> HHHHHHSSGLVPRGSH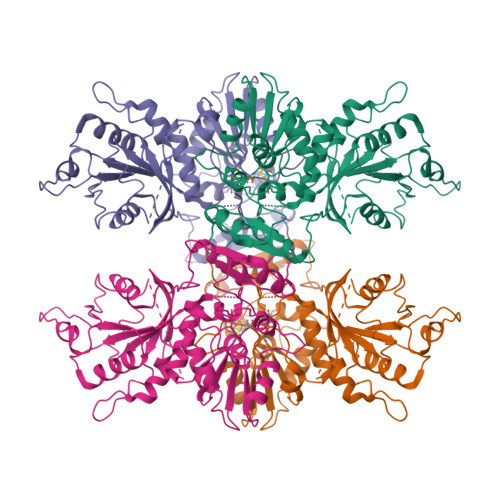MLEDPRRYTMRLPDAGFRRYIVVAGRRNVGKSSFMNALVGQNVSIVSDYAGTTTDPVYKSMELHPIGPVTLVDTPGLDDVGELGRLRVEKARRVFYRADCGILVTDSAPTPYEDDVVNLFKEMEIPFVVVVNKIDVLGEKAEELKGLYESRYEAKVLLVSALQKKGFDDIGKTISEILPGDEEIPYLGDLIDGGDLVILVVPIDLGAPKGRLIMPQVHAIREALDREAIALVVKERELRYVMENIGMKPKLVITDSQVAMKVASDVPEDVELTTFSIVESRYRGDLAYFVESVRKIEELEDGDTVVIMEGCTHRPLTEDIGRVKIPRWLVNHTGAQLNFKVIAGKDFPDLEEIENAKLIIHCGGCILNRSAMMRRVRMAKRLGIPMTNYGVTISYLHGVLERAIRPF>[8x]ELYSIPEDQEPEDQEPEEPTPAPWARLWALQDGFANLECVNDNYWFGRDKSCEYCFDEPLLKRTDKYRTYSKKHFRIFREVGPKNSYIAYIEDHSGNGTFVNTELVGKGKRRPLNNNSE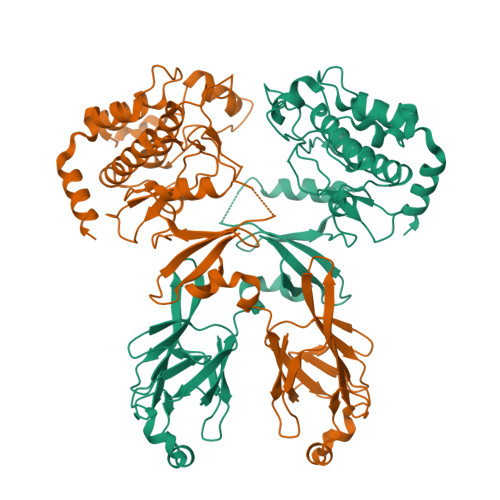IALSLSRNKVFVFFDLTVDDQSVYPKALRDEYIMSKTLGSGACGEVKLAFERKTCKKVAIRIISKRKFAIGSAREADPALNVETEIEILKKLNHPCIIKIKNFFDAEDYYIVLELMEGGELFDKVVGNKRLKEATCKLYFYQMLLAVQYLHENGIIHRDLKPENVLLSSQEEDCLIKITDFGHSKILGETSLMRTLCGTPTYLAPEVLVSVGTAGYNRAVDCWSLGVILFICLSGYPPFSEHRTQVSLKDQITSGKYNFIPEVWAEVSEKALDLVKKLLVVDPKARFTTEEALRHPWLQDEDMKRKFQDLLSEENESTALPQVL> MSTIGAVDILNQKTITSEVAASVTSKYLQSTFSKGNTSHIEDKRFIHVSSRSHSRFTSTPITPNEILSLKFHVSGSSMAYSRMDGSLTVWFIKDASFDKSVEVYIPDCCGSDKLATDLSWNPTSLNQIAVVSNSSEISLLLINEKSLTASKLRTLSLGSKTKVNTCLYDPLGNWLLAATKSEKIYLFDVKKDHSSVCSLNISDISQEDNDVVYSLAWSNGGSHIFIGFKSGYLAILKAKHGILEVCTKIKAHTGPITEIKMDPWGRNFITGSIDGNCYVWNMKSLCCELIINDLNSAVTTLDVCHLGKILGICTEDEMVYFYDLNSGNL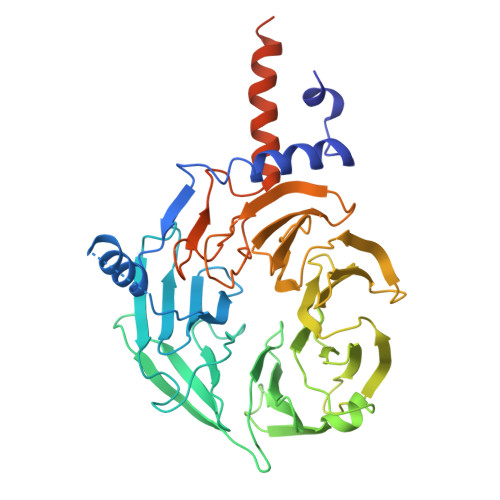LHSKSLANYKTDPVLKFYPDKSWYIMSGKNDTLSNHFVKNEKNLITYWKDMFDNTMIEKRRKNNGGGNNHNKRTSKNTDRIGKDRPSRFNSKK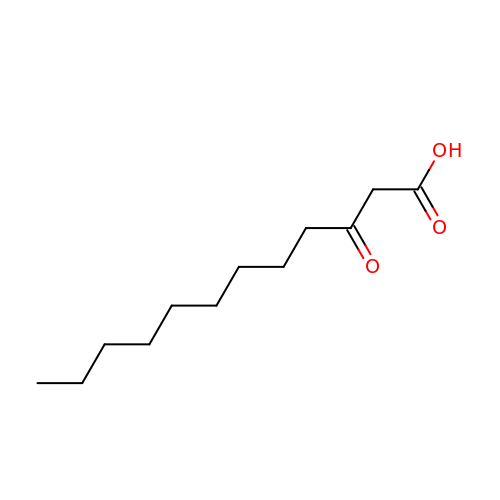3-OXODODECANOIC ACID | C12 H22 O3 | DZHSPYMHDVROSM-UHFFFAOYSA-N> EVANPEHYIKHPLQNRWALWFFKNDKSKTWQANLRLISKFDTVEDFWALYNHIQLSSNLMPGCDYSLFKDGIEPMWEDEKNKRGGRWLITLNKQQRRSDLDRFWLETLLCLIGESFDDYSDDVCGAVVNVRAKG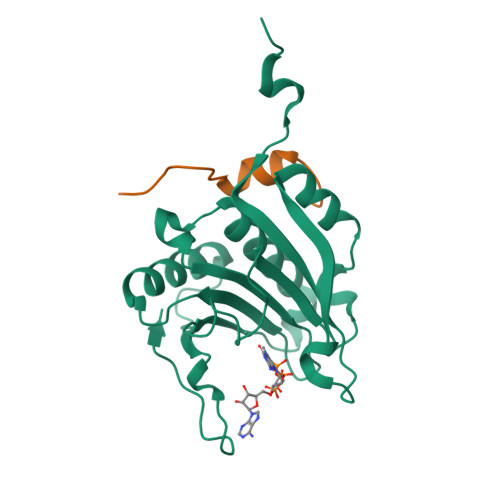DKIAIWTTECENREAVTHIGRVYKERLGLPPKIVIGYQSHADTATKSGSTTKNRFVV;> PGGTRIIYDRKFLMECRNSP>GAMGNPLRKFKLVFLGEQSVGKTSLITRFMYDSFDNTYQATIGIDFLSKTMYLEDRTVRLQLWDTAGLERFRSLIPSYIRDSTVAVVVYDITNVNSFQQTTKWIDDVRTERGSDVIIMLVGNKTDLADKRQVSIEEGERKAKELNVMFIETSAKAGYNVKQLFRRVAAALPGMESTQDRSREDMIDIKLEK[2x];>GAMEQWCSERLDNQKELMEELYEEKLKILKESLTTFYQEQIQERDEKIEELETLLQEAKQQPAAQQ[2x]

One of the main functions of RAB GTPases is to recruit actin- or MT- based motors on transport carriers, allowing them to move along cytoskeletal tracks. This is the case for RAB6, the most abundant RAB at the Golgi that regulates several transport steps at the Golgi as well as Golgi homeostasis. Two closely related RAB6 isoforms, RAB6A and RAB6A′ are present on Golgi/TGN membranes. The interaction between RAB6 and Myosin II is critical for the fission of RAB6-positive transport carriers from Golgi/TGN membranes. Here, we show that KIF20A is also involved in the fission process.

To further characterize this interaction, we solved the crystal structure of the complex between RAB6 and KIF20A. The RAB6:KIF20A structure reveals that the 603–645 residues of KIF20A represent the RBD. KIF20A-RBD is a dimer composed of two parallel alpha helices that form a right-handed coiled-coil additionally stabilized by an inter-helical cysteine bridge. Both RBD helices participate in RAB6 binding, two RAB6 molecules binding at opposite sides of the dimer. The RAB6:KIF20A interface is formed by complementary surfaces of the partners that mediate hydrophobic and polar contacts between the molecules. KIF20A K629 and S630 residues are located in the central part of the RAB6-binding site and form polar contacts with the partner. Prediction based on the structure indicates that substitution of these polar residues by bulky hydrophobic residues should substantially alter the RAB6-binding site. Indeed, the KIF20A (529–665) fragment with K629W and S630W mutations lost its capacity to interact with RAB6 Q72L by yeast two-hybrid. A myc-tagged version of the KIF20A-529-665-K629W-S630W fragment overexpressed in HeLa cells remained mostly cytosolic in contrast to the Golgi-localized wild-type form, demonstrating the importance of the RAB6:KIF20A direct interaction for KIF20A recruitment to Golgi. The mutations do not affect KIF20A-RBD dimerization and importantly its ability to interact with the tail domain of Myosin II.> EAERVRVFHKQAFEYISIALRIDEDEKAGQK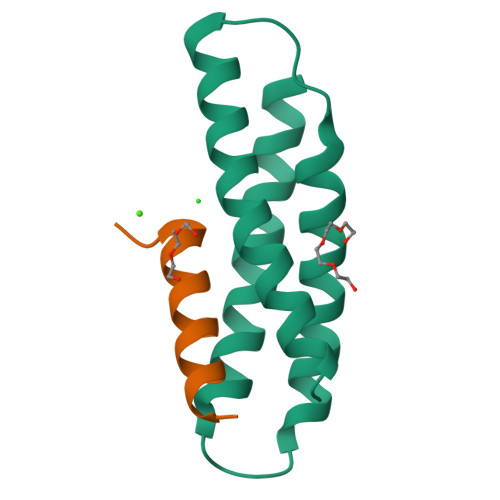EQAVEWYKKGIEELEKGIAVIVTGQGEQCERARRLQAKMMTNLVMAKDRLQLL;> TSASEDIDFDDLSRRFEELKKKT>ASDHQTQAGKPQPLNPKIIIFEQENFQGHSHELSGPCPNLKETGMEKAGSVLVQAGPWVGYEQANCKG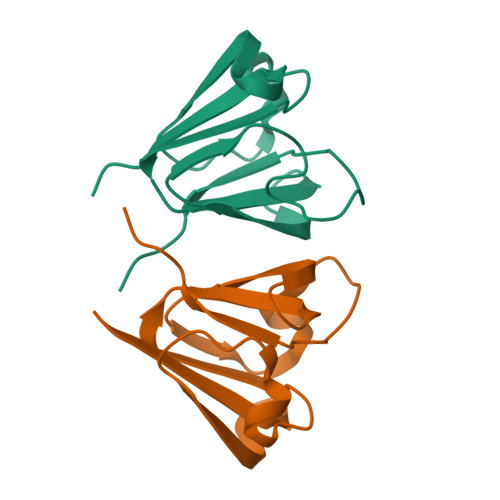EQFVFEKGEYPRWDSWTSSRRTDSLSSLRPIKVDSQEH[2x]> MIEIKDKQLTGLRFIDLFAGLGGFRLALESCGAECVYSNEWDKYAQEVYEMNFGEKPEGDITQVNEKTIPDHDILCAGFPCQAFSISGKQKGFEDSRGTLFFDIARIVREKKPKVVFMENVKNFASHDNGNTLEVVKNTMNELDYSFHAKVLNALDYGIPQKNERIYMICFRNDLNIQNFQFPKPFELNTFVKDLLLPDSEVEHLVIDRKDLVMTNQEIEQTTPKTVRLGIVGKGGQGERIYSTRGIAITLSAYGGGIFAKTGGYLVNGKTRKLHPRECARVMGYPDSYK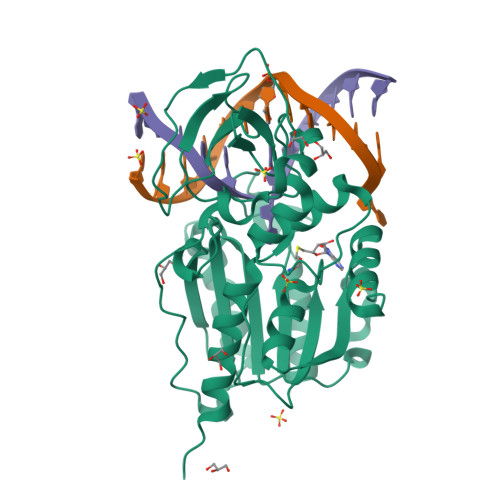VHPSTSQAYKQFGNSVVINVLQYIAYNIGSSLNFKPY> MGASARLLRAVIMGAPGSGKGTVSSRITTHFELKHLSSGDLLRDNMLRGTEIGVLAKAFIDQGKLIPDDVMTRLALHELKNLTQYSWLLDGFPRTLPQAEALD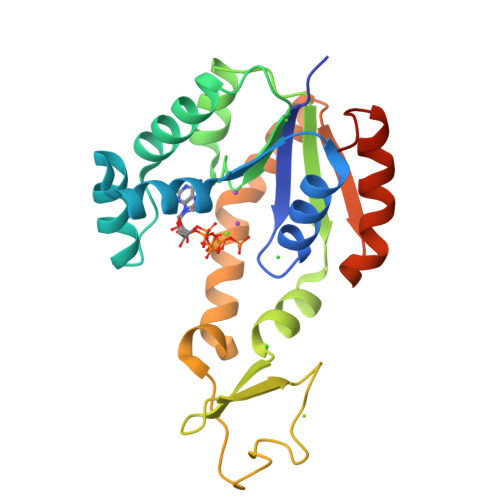RAYQIDTVINLNVPFEVIKQRLTARWIHPASGRVYNIEFNPPKTVGIDDLTGEPLIQREDDKPETVIKRLKAYEDQTKPVLEYYQKKGVLETFSGTETNKIWPYVYAFLQTKVPQRSQKASVTP>HPETLVKVKDAEDQLGARVGYIELDLNSGKILESFRPEERFPMMSTFKVLLCGAVLSRIDAGQEQLGRRIHYSQNDLVEYSPVTEKHLTDGMTVRELCSAAITMSDNTAANLLLTTIGGPKELTAFLHNMGDHVTRLDRWEPELNEAIPNDERDTTMPAAMATTLRKLLTGELLTLASRQQLID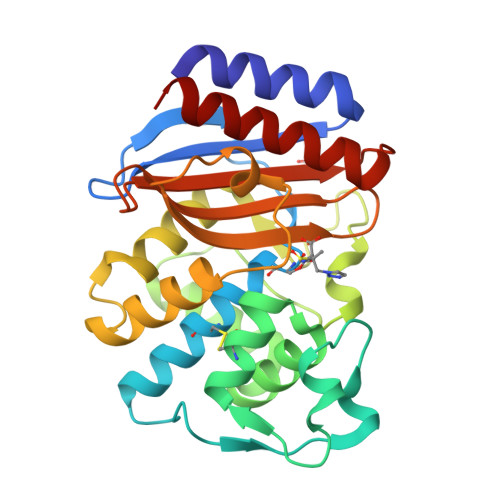WMEADKVAGPLLRSALPAGWFIADKSGAGERGSRGIIAALGPDGKPSRIVVIYTTGSQATMDERNRQIAEIGASLIKHW[6x]> MGSKYSKATNSINDALSSSYLVPFESYRVPLVDLEEATNNFDHKFLIGHGVFGKVYKGVLRDGAKVALKRRTPES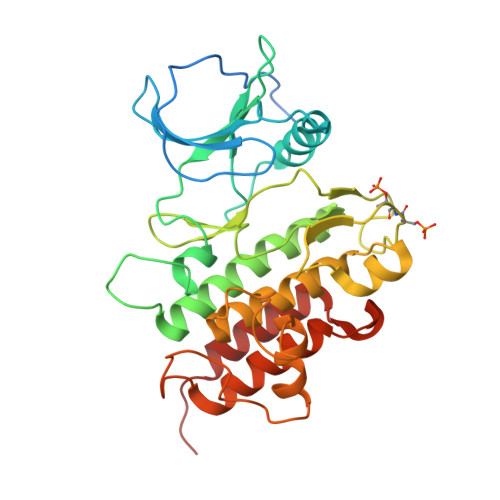SQGIEEFETEIETLSFCRHPHLVSLIGFCDERNEMILIYKYMENGNLKRHLYGSDLPTMSMSWEQRLEICIGAARGLHYLHTRAIIHRDVKSINILLDENFVPKITDFGISKKGTELDQTHLSTVVKGTLGYIDPEYFIKGRLTEKSDVYSFGVVLFEVLCARSAIVQSLPREMVNLAEWAVESHNNGQLEQIVDPNLADKIRPESLRKFGDTAVKCLALSSEDRPSMGDVLWKLEYALRLQESVI> CGN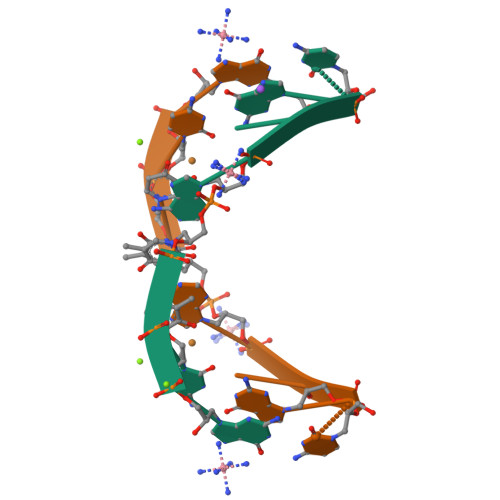AXNCG2-acetamido-2,5-dideoxy-6-O-phosphono-D-lyxo-hexose | C8 H16 N O8 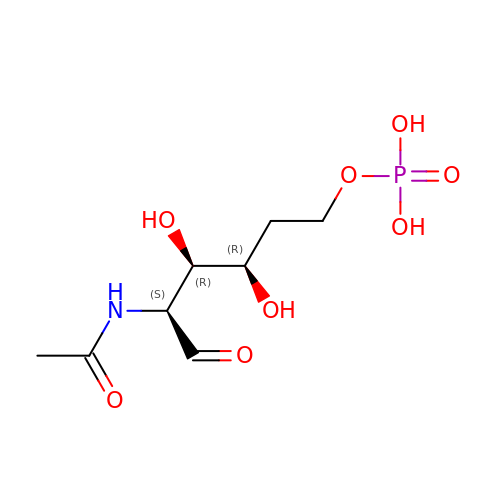P | SJEDNRVDWMBCDP-BWZBUEFSSA-N> LMYYESLTKQYPVSKTIRNELIPIGKTLDNIRQNNILESDVKRKQNYEHVKGILDEYHKQLINEALDNCTLPSLKIAAEIYLKNQKEVSDREDFNKTQDLLRKEVVEKLKAHENFTKIGKKDILDLLEKLPSISEDDYNALESFRNFYTYFTSYNKVRENLYSDKEKSSTVAYRLINENFPKFLDNVKSYRFVKTAGILADGLGEEEQDSLFIVETFNKTLTQDGIDTYNSQVGKINSSINLYNQKNQKANGFRKIPKMKMLYKQILSDREESFIDEFQSDEVLIDNVESYGSVLIESLKSSKVSAFFDALRESKGKNVYVKNDLAKTAMSNIVFENWRTFDDLLNQEYDLANENKKKDDKYFEKRQKELKKNKSYSLEHLCNLSEDSCNLIENYIHQISDDIENIIINNETFLRIVINEHDRSRKLAKNRKAVKAIKDFLDSIKVLERELKLINSSGQELEKDLIVYSAHEELLVELKQVDSLYNMTRNYLTKKPFSTEKVKLNFNRSTLLNGWDRNKETDNLGVLLLKDGKYYLGIMNTSANKAFVNPPVAKTEKVFKKVDYKLLPVPNQMLPKVFFAKSNIDFYNPSSEIYSNYKKGTHKKGNMFSLEDCHNLIDFFKESISKHEDWSKFGFKFSDTASYNDISEFYREVEKQGYKLTYTDIDETYINDLIERNELYLFQIYNKDFSMYSKGKLNLHTLYFMMLFDQRNIDDVVYKLNGEAEVFYRPASISEDELIIHKAGEEIKNKNPNRARTKETSTFSYDIVKDKRYSKDKFTLHIPITMNFGVDEVKRFNDAVNSAIRIDENVNVIGIDRGERNLLYVVVIDSKGNILEQISLNSIINKEYDIETDYHALLDEREGGRDKARKDWNTVENIRDLKAGYLSQVVNVVAKLVLKYNAIICLEDLNFGFKRGRQKVEKQVYQKFEKMLIDKLNYLVIDKSREQTSPKELGGALNALQLTSKFKSFKELGKQSGVIYYVPAYLTSKIDPTTGFANLFYMKCENVEKSKRFFDGFDFIRFNALENVFEFGFDYRSFTQRACGINSKWTVCTNGERIIKYRNPDKNNMFDEKVVVVTDEMKNLFEQYKIPYEDGRNVKDMIISNEEAEFYRRLYRLLQQTLQMRNSTSDGTRDYIISPVKNKREAYFNSELSDGSVPKDADANGAYNIARKGLWVLEQIRQKSEGEKINLAMTNAEWLEYAQTHLL;> MYYESLTKQYPVSKTIRNELIPIGKTLDNIRQNNILESDVKRKQNYEHVKGILDEYHKQLINEALDNCTLPSLKIAAEIYLKNQKEVSDREDFNKTQDLLRKEVVEKLKAHENFTKIGKKDILDLLEKLPSISEDDYNALESFRNFYTYFTSYNKVRENLYSDKEKSSTVAYRLINENFPKFLDNVKSYRFVKTAGILADGLGEEEQDSLFIVETFNKTLTQDGIDTYNSQVGKINSSINLYNQKNQKANGFRKIPKMKMLYKQILSDREESFIDEFQSDEVLIDNVESYGSVLIESLKSSKVSAFFDALRESKGKNVYVKNDLAKTAMSNIVFENWRTFDDLLNQEYDLANENKKKDDKYFEKRQKELKKNKSYSLEHLCNLSEDSCNLIENYIHQISDDIENIIINNETFLRIVINEHDRSRKLAKNRKAVKAIKDFLDSIKVLERELKLINSSGQELEKDLIVYSAHEELLVELKQVDSLYNMTRNYLTKKPFSTEKVKLNFNRSTLLNGWDRNKETDNLGVLLLKDGKYYLGIMNTSANKAFVNPPVAKTEKVFKKVDYKLLPVPNQMLPKVFFAKSNIDFYNPSSEIYSNYKKGTHKKGNMFSLEDCHNLIDFFKESISKHEDWSKFGFKFSDTASYNDISEFYREVEKQGYKLTYTDIDETYINDLIERNELYLFQIYNKDFSMYSKGKLNLHTLYFMMLFDQRNIDDVVYKLNGEAEVFYRPASISEDELIIHKAGEEIKNKNPNRARTKETSTFSYDIVKDKRYSKDKFTLHIPITMNFGVDEVKRFNDAVNSAIRIDENVNVIGIDRGERNLLYVVVIDSKGNILEQISLNSIINKEYDIETDYHALLDEREGGRDKARKDWNTVENIRDLKAGYLSQVVNVVAKLVLKYNAIICLEDLNFGFKRGRQKVEKQVYQKFEKMLIDKLNYLVIDKSREQTSPKELGGALNALQLTSKFKSFKELGKQSGVIYYVPAYLTSKIDPTTGFANLFYMKCENVEKSKRFFDGFDFIRFNALENVFEFGFDYRSFTQRACGINSKWTVCTNGERIIKYRNPDKNNMFDEKVVVVTDEMKNLFEQYKIPYEDGRNVKDMIISNEEAEFYRRLYRLLQQTLQMRNSTSDGTRDYIISPVKNKREAYFNSELSDGSVPKDADANGAYNIARKGLWVLEQIRQKSEGEKINLAMTNAEWLEYAQTHLL

Cas12a is a programmable nuclease for adaptive immunity against invading nucleic acids in CRISPR–Cas systems. Among the Cas12a orthologs, Lachnospiraceae bacterium MA2020 (Lb2) Cas12a is the smallest in molecular weight and recognizes a short spacer (14 nt) for cleavage and the creation of indels with high fidelity. Typically, Cas12a exhibits a bilobed architecture: a recognition lobe (the REC1 and REC2 domains), and a nuclease (NUC) lobe (the WED, PI, RuvC, BH, and Nuc domains) for cleaving nucleic acids. We demonstrate that apo Lb2Cas12a assumes a unique, elongated conformation, whereas the Lb2Cas12a+crRNA binary complex exhibits a compact conformation that subsequently rearranges to a semi-open conformation in the Lb2Cas12a+crRNA+DNA ternary complex.

Strikingly, both apo and RNA-bound Lb2Cas12a are present in the asymmetric unit of the crystal. The 20 nucleotides of the crRNA in the complex are well defined in the electron density map. In apo Lb2Cas12a, the N-terminal REC1 and REC2 domains (REC lobe) and the C-terminal wedge (WED), RuvC, and Nuc domains (NUC lobe) are arranged in an elongated conformation, with the REC1 domain and Nuc domain at each end. Two flexible loops (Asn33–Asn45 and Lys478–Thr498) connect the REC and NUC lobes. The overall 3D structure of the Lb2Cas12a+crRNA binary complex adopts a triangular, compact conformation. The REC and NUC lobes lie adjacent to each other in 3D space, creating a positively charged cavity in the center. Superposition of the apo Lb2Cas12a and Lb2Cas12a+crRNA binary complex structures demonstrates a 103° rotation of the REC lobe with respect to the α-helix of the WED-I domains of the crRNA complex in its compact conformation. Residues from the region Met493–Leu523 of the WED domain participate in major conformational changes to facilitate the structural rearrangements associated with this rotation. The flexible loop (Leu477–Lys493) connecting the REC and RuvC domains of apo Lb2Cas12a transforms into an α-helix in the compact conformation, folding back at the C-terminus of the REC2 domain. Significantly, the loop-turned-α-helix (Leu477–Lys493) harbors a hydrophobic patch that interacts with Trp871, linking the REC and NUC lobes through the BH and RuvC II suspension helix.>[8x]SMTEIRVHQGDLPNLDNYRIDAVAVDTETLGLQPHRDRLCVVQLSSGDGTADVIQIAKGQKSAPNLVRLLSDRDITKIFHFGRFDLAILAHTFGVMPDVVFCTKIASKLTRTYTDRHGLKEICGELLNVNISKQQQSSDWAAETLSRAQIEYAASDVLYLHRLKDIFEERLKREERESVAKACFQFLPMRANLDLLGWSEIDIFAHS

Orn and NrnC are 3′–5′ exonucleases with a DnaQ fold containing the catalytic DEDD motif, a domain that is common in enzymes that act on nucleic acids. Notably, Orn (and its eukaryotic ortholog REXO2) or NrnC activity is critical for cellular growth, rendering them unique amongst the exoribonucleases known to date. Through quantitative structure-function analyses, we show here that NrnC-type RNases share this narrow substrate length preference with Orn. The structures confirm an octameric assembly as a conserved feature of NrnC-type RNases.

To answer this question, we determined crystal structures of wild-type B. henselae and B. melitensis NrnC (NrnCBh and NrnCBm, respectively) bound to pGG and, in the case of NrnCBm, also in the substrate-free state. The diribonucleotide pGG is bound to all eight active sites of the NrnCBh octameric assembly. The active sites face the center of the central cavity formed by the NrnC octamer, positioned mid-way of each ring. In this crystallographic state, the residues of the catalytic DEDDy signature motif (D25, E27, D84, D155, Y151) are primed for accepting divalent metal ions for nucleotide hydrolysis. The side chain of Y151 coordinates a water molecule, which likely serves as the attacking nucleophile in the reaction. The structure also reveals the molecular basis for substrate coordination. Reminiscent of Orn’s active site, the bases of the diribonucleotide are splayed apart by a leucine residue, or L-wedge (L31). Continuing with the parallels to Orn, the 5′ phosphate of pGG is coordinated by several residues forming a ‘phosphate cap,’ in this case basic residues H79, K103, and H205, the latter being the second to last residue of the protein, contributed from a subunit from the adjacent ring. The specific motifs coordinating the substrate are invariable in NrnC orthologs, in contrast to the exterior surface with overall lower conservation, and culminate in a length-restricted active site that appears optimized for diribonucleotides. A comparison with the structurally related Rrp6 exonuclease subunit of the exosome bound to a longer RNA substrate supports this notion as residues K103 and H205 of NrnC’s phosphate cap directly block the path for longer substrates (Wasmuth et al., 2014).> GPAKQYDSVECPFCDEVSKYEKLAKIGQGTFGEVFKARHRKTGQKVALKKVLMENEKEGFPITALREIKILQLLKHENVVNLIEICRTKASPYNRCKGSIYLVFDFCEHDLAGLLSNVLVKFTLSEIKRVMQMLLNGLYYIHRNKILHRDMKAANVLITRDGVLKLADFGLARAFSLAKNSQPNRYTNRVVTLWYRPPELLLGERDYGPPIDLWGAGCIMAEMWTRSPIMQGNTEQHQLALISQLCGSITPEVWPNVDNYELYEKLELVKGQKRKVKDRLKAYVRDPYALDLIDKLLVLDPAQRIDSDDALNHDFFWSDPMPSDLKGMLST;> GPEGERKNNNKRWYFTREQLENSPSRRFGVDPDK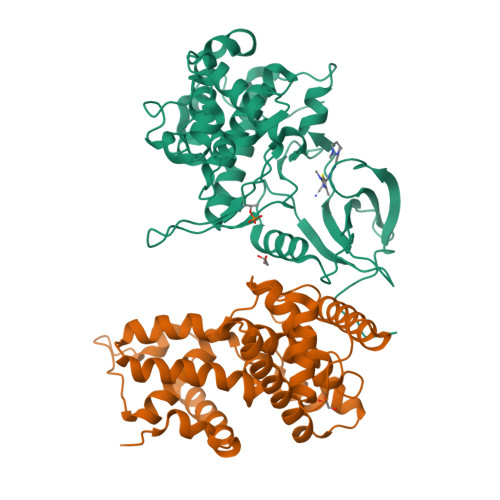ELSYRQQAANLLQDMGQRLNVSQLTINTAIVYMHRFYMIQSFTRFPGNSVAPAALFLAAKVEGQPKKLEHVIKVAHTCLHPQESLPDTRSEAYLQQVQDLVILESIILQTLGFELTIDHPHTHVVKCTQLVRASKDLAQTSYFMATNSLHLTTFSLQYTPPVVACVCIHLACKWSNWEIPVSTDGKHWWEYVDATVTLELLDELTHELLQILEKTPNRLKRIWNWR>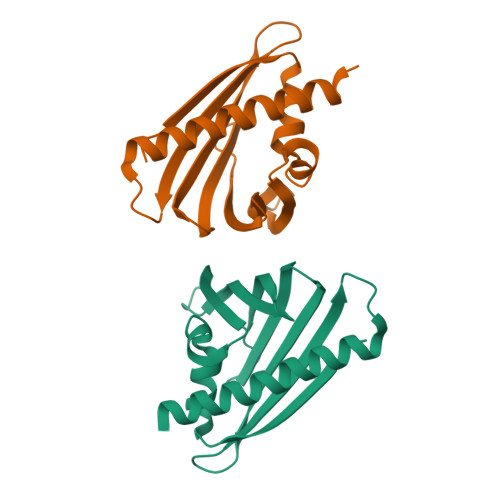[2x]GHMVSKTVEVAASAETITSIVSDFEAYPQWNPEIKGCWILARYNDGRPSQLRLDVEIQGQSGVFITAVYYPAENQIFTMLQQGDHFTKQEQRFSIVPLGPDSTLLQVDLDVEVKLPVPGPMVKKLAGETLEHLAKALEGRVEQLTQS>PDAPQIAAKGYVLMDYHSGKVLAEKEMDTKLSPASLTKMMTSYVIGQEVKRGNISLNDDVVISKNAWAKNFPDSSKMFVEVGTTVKVSDLNRGIIIQSGNDACVAMAEHVAGTEDAFVDLMNAWASSLGMKNSHFTNSHGLDDPNLYSTPYDLALLGQALIRDVPEEYAIYSEQKFTYNGITQYNRNGLLWDKSMNVDGIKTGHTSGAGYNL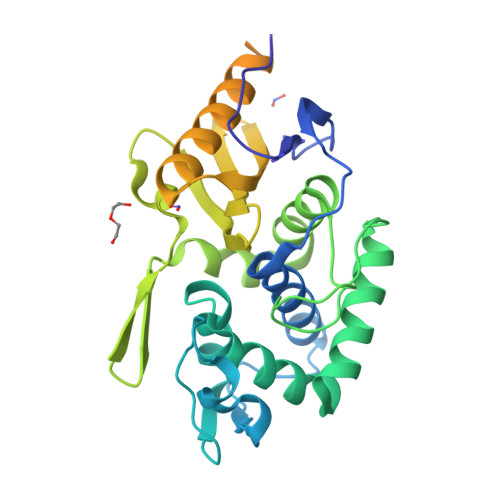VSSATEGNMRLVAVVMGTDNENARKAESKKLLSYGFRFFETVAPHKAGETFVNETIWMGDKDTIALGVDKDTYVTLPRGQAKDLTASFVLEKQLKAPLKKGDIVGTLYYQLAGNDIAQYPLLALEDVQE[3x]> MSDTEKDKDVPMVDSHEATEEPPTTSTNTPSFPHLAQEQAKEESATLGAEVAHKKINYEQEAQKLEEKALRFLAKQTHPVIIPSFASWFDISKIHEIEKRSNPDFFNDSSRFKTPKAYKDTRNFIINTYRLSPYEYLTITAVRRNVAMDVASIVKIHAFLEKWGLINYQID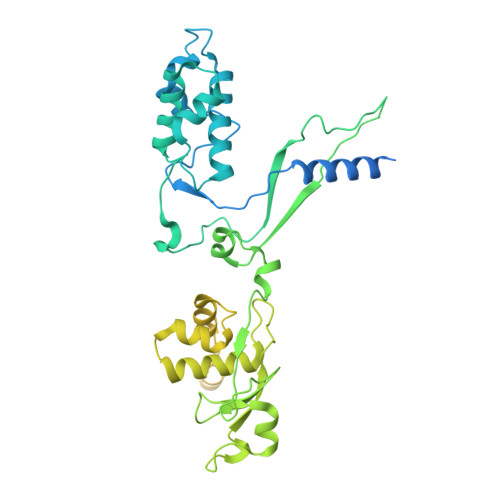PRTKPSLIGPSFTGHFQVVLDTPQGLKPFLPENVIKQEVEGGDGAEPQVKKEFPVNLTIKKNVYDSAQDFNALQDESRNSRQIHKVYICHTCGNESINVRYHNLRARDTNLCSRCFQEGHFGANFQSSDFIRLENNGNSVKKNWSDQEMLLLLEGIEMYEDQWEKIADHVGGHKRVEDCIEKFLSLPIEDNYIREVVGSTLNGKGGDSRDGSVSGSKLMECVNDAVQTLLQGDDKLGKVSDKSREISEKYIEESQAIIQELVKLTMEKLESKFTKLCDLETQLEMEKLKYVKESEKMLNDRLSLSKQILDLNKSLEELNVSKKLVLISEQVDSGIQLVEKDQEGDDEDGNTATGHGVKRVGKEGEEVGEGDSIAKLQPQVYKPWSL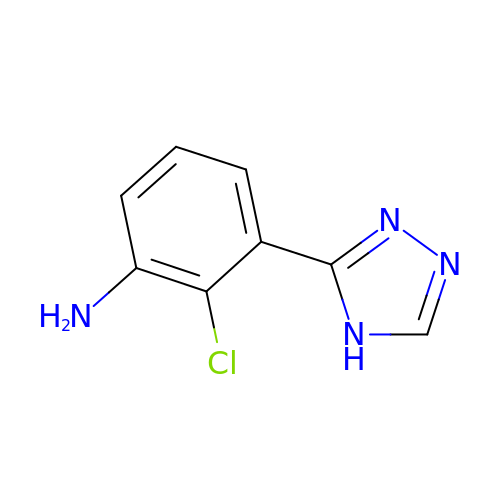2-chloranyl-3-(4~{H}-1,2,4-triazol-3-yl)aniline | C8 H7 Cl N4 | RWTMHFLYHAPAAV-UHFFFAOYSA-N>[8x]SLSSVKDFPKIKAIRSFIIGGVGSGGDYHNVKGGHWLIDSDISTPASKWEQYKKSRTSWGINVLGSFLVEIEATDGTVGFATGFGGPPAC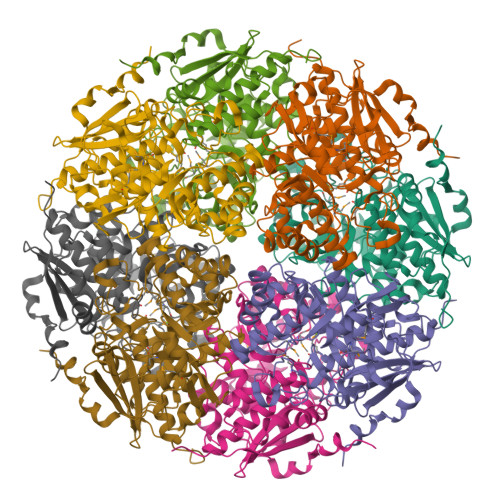WLVHQHFERFLIGADPRNTNLLFEQMYRASMFYGRKGLPIAVISVIDLALWDLLGKVRNEPVYRLIGGATKERLDFYCTGPEPTAAKAMGFWGGKVPLPFCPDDGHEGLRKNVEFLRKHREAVGPDFPIMVDCYMSLNVSYTIELVKACLDLNINWWEECLSPDDTDGFALIKRAHPTVKFTTGEHEYSRYGFRKLVEGRNLDIIQPDVMWLGGLTELLKVAALAAAYDVPVVPHASGPYSYHFQISQPNTPFQEYLANSPDGKSVLPVFGDLFIDEPIPTKGYLTTADLDKPGFGLTINPAARAKLIPSDYLFKVPEIPQNLSTGKEIKSNEQPDKPNGTLDSLAAKVESLTTSTSSEGHHHHH>SKPFSVPVLTVEEMTNSRFPIPLEKLFTGPSSAFVVQPQNGRCTTDGVLLGTTQLSPVNICTFRGDVTHITGSRNYTMNLASQNWNDYDPTEEIPAPLGTPDFVGKIQGVLTQTTRTDGSTRGHKATVYTGSADFAPKLGRVQFETDTDRDFEANQNTKFTPVGVIQDGGTTHRNEPQQWVLPSYSGRNTHNVHLAPAVAPTFPGEQLLFFRSTMPGCSGYPNMDLDCLLPQEWVQYFYQEAAPAQSDVALLRFVNPDTGRVLFECKLHKSGYVTVAHTGQHDLVIPPNGYFRFDSWVNQFYTLAPM[2x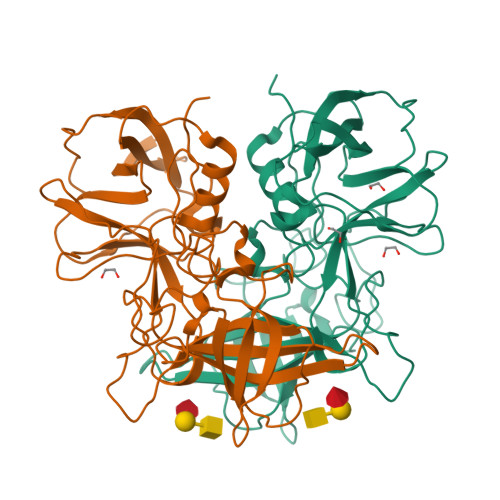]> MAKKTSGRGKLPPGPTPLPVIGNILQIGIKDISKSLTNLSKVYGPVFTLYFGLKPIVVLHGYEAVKEALIDLGEEFSGRGIFPLAERANRGFGIVFSNGKKWKEIRRFSLMTLRNFGMGKRSIEDRVQEEARCLVEELRKTKASPCDPTFILGCAPCNVICSIIFHKRFDYKDQQFLNLMEKLNENIKILSSPWIQICNNFSPIIDYFPGTHNKLLKNVAFMKSYILEKVKEHQESMDMNNPQDFIDCFLMKMEKEKHNQPSEFTIESLENTAVDLFGAGTETTSTTLRYALLLLLKHPEVTAKVQEEIERVIGRNRSPCMQDRSHMPYTDAVVHEVQRYLDLLPTSLPHAVTCDIKFRNYLIPKGTTILISLTSVLHDNKEFPNPEMFDPHHFLDEGGNFKK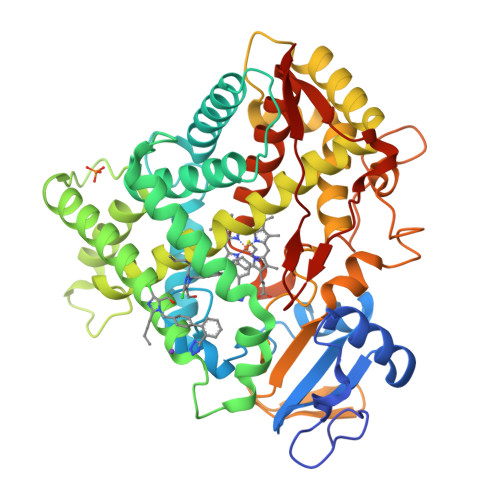SKYFMPFSAGKRICVGEALAGMELFLFLTSILQNFNLKSLVDPKNLDTTPVVNGFASVPPFYQLCFIPIHHHH> MAEIGTGFPFDPHYVEVLGERMHYVDVGPRDGTPVLFLHGNPTSSYVWRNIIPHV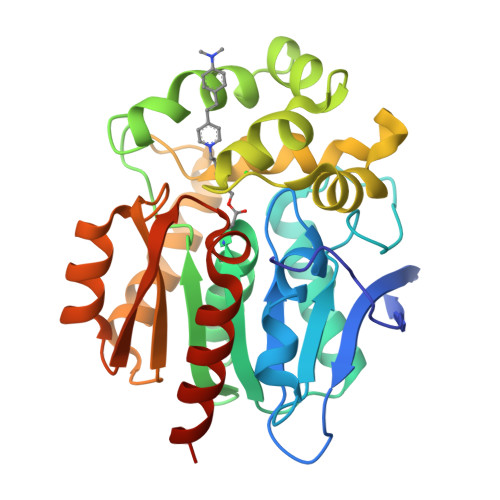APTHRCIAPDLIGMGKSDKPDLGYFFDDHVRFMDAFIEALGLEEVVLVIHDWGSALGFHWAKRNPERVKGIAFMEFIRPIPTWDEWPEFARETFQAFRTTDVGRKLIIDQNVFIEGTLPMGVVRPLTEVEMDHYREPFLNPVDREPLWRFPNELPIAGEPANIVALVEEYMDWLHQSPVPKLLFWGTPGVLIPPAEAARLAKSLPNCKAVDIGPGLNLLQEDNPDLIGSEIARWLSTLEHHHHHH>[2x]ISEFEKGYQSQLYTEMVGINNISKQFILKNPLDDNQTIKSKLERFVSGYKMNPKIAEKYNVSVHFVNKEKPRAYSLVGVPKTGTGYTLSVWMNSVG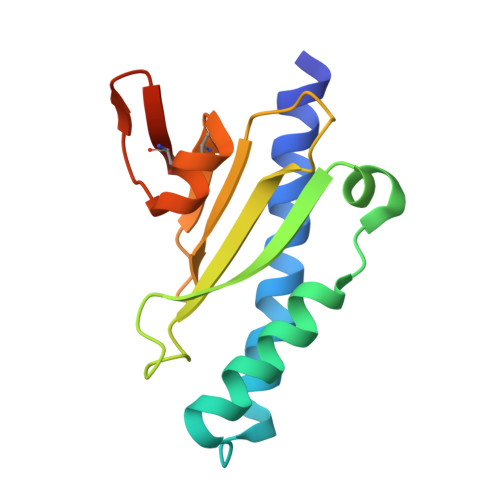DGYKCRDAASARAHLETLSSDVGCEAFSNRKK> MRPAQTNQFDYVKIGLASPERIRQWGERTLPNGQVVGEVTKPETINYRTLKPEMDGLFCERIFG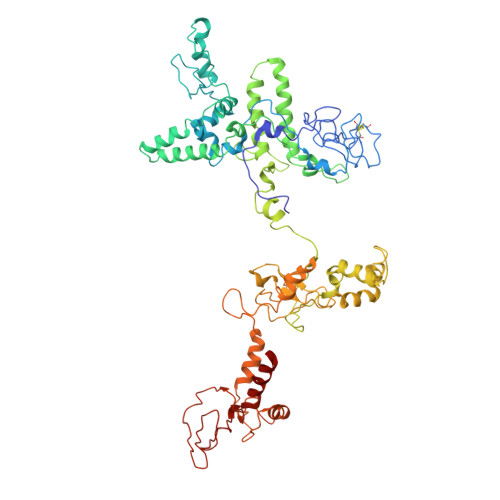PAKDWECHCGKYKRVRHRGIVCERCGVEVTESRVRRHRMGYIKLAAPVAHVWYLKGIPSYISILLDMPLRDVEQIVYFNSYVVLSPGNAETLTYKQLLSEDQWLEIEDQIYSEDSQLQGVEVGIGAEALLRLLADINLEQEAESLREEIGSAKGQKRAKLIKRLRVIDNFIATGSKPEWMVMTVIPVIPPDLRPMVQLDGGRFATSDLNDLYRRVINRNNRLARLQEILAPEIIVRNEKRMLQEAVDALIDNGRRGRTVVGANNRPLKSLSDIIEGKQGRFRQNLLGKRVDYSGRSVIVVGPKLKIHQCGLPREMAIELFQPFVINRLIRSGMVNNIKAAKKLISRNDPSVWDVLEEVIEGHPVMLNRAPTLHRLGIQAFEPILVEGRAIQLHPLVCPAFNADFDGDQMAVHVPLSLESQAEARLLMLASNNILSPATGRPIITPSQDMVLGAYYLTAENPGATKGAGKYFASLDDVIMAFQQEQIDLHAYVYVRFDGDVESDQPDTEPVKVTTNEDGSRTVLYKYRRVREDAQGNVISQYIYTTPGRVIYNKAIQEALAS> MSLQLRSRAAFKLEFLLDRYRVVRKGDAVIEIGSSPGGWTQVLNSLARKIISIDLQEME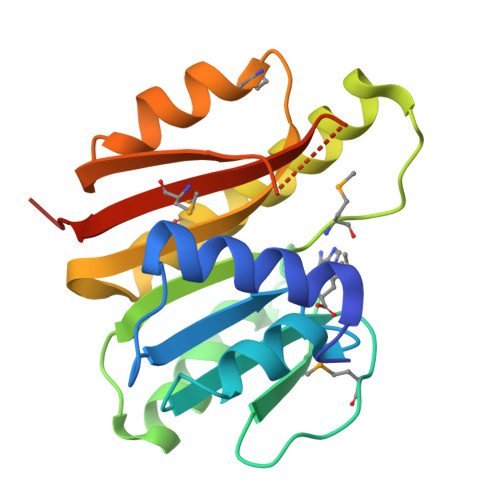EIAGVRFIRCDIFKETIFDDIDRALREEGIEKVDDVVSDAMAKVSGIPSRDHAVSYQIGQRVMEIAVRYLRNGGNVLLKQFQGDMTNDFIAIWRKNFSSYKISKPPASRGSSSEIYIMFFGFKAEGHHHHHH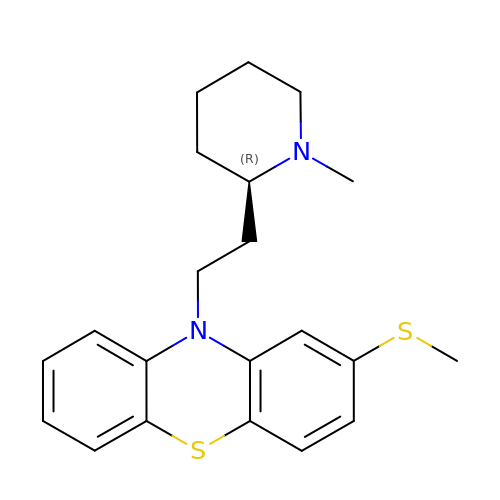10-{2-[(2R)-1-methylpiperidin-2-yl]ethyl}-2-(methylsulfanyl)-10H-phenothiazine | C21 H26 N2 S2 | KLBQZWRITKRQQV-MRXNPFEDSA-N> YDPFKYVETVFVVDKAMVTKYNGDLDKIKTKMYEAANNMNEMYRYMFFRVVMVGLIIWTEEDKITVKPDVDYTLNAFAEWRKTYLLAEKKHDNAQLITGIDFRGSIIGYAYIGSM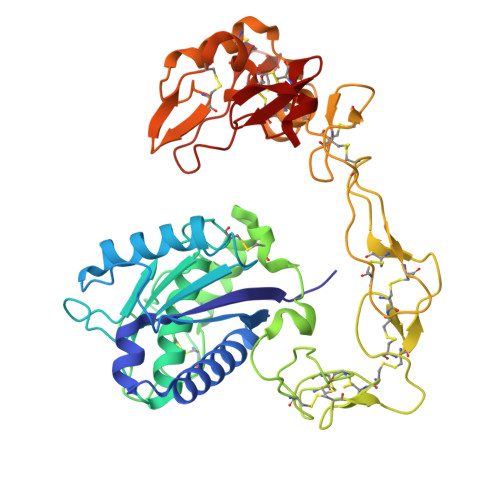CHPKRSVGIIQDYSPINLVLAVIMAHEMGHNLGIHHDDGYCYCGGYPCIMGPSISPEPSKFFSNCSYIQCWDFIMNHNPECIDNEPLGTDIISPPLCGNELLEVGEECDCGTPENCQNPCCDAATCKLKSGSQCGHGKCCEQCKFRTSGTECRASMSECDPAEHCTGQSSECPADVFHKNGEPCLDNYGYCYNGNCPIMYHQCYALFGADIYEAEDSCFESNKKGNYYGYCRKENGKKIPCASEDVKCGRLYCKDDSPGQNNPCKMFYSNDDEHKGMVLPGTKCADGKVCSNGHCVDVTTAY> WNSRYSYNQLKNKDSLIMFLVEIFRSLFVSNCIDKNIDNVLLSIEEMFIDHYYNPQHSRLKYLIDDVGIFFTKLPITKAFHTYNKKYRITKRLYAPPTFNEVRHILNLAQILSLEEGLDLLTFDANETLYPDGHDFNDEVLASYISCLLKKMNIAIVTAASYNNDAEKYQKRLENLLKYFSKHNIKDGSYKNFYVMGGESNYLFKCNEEATL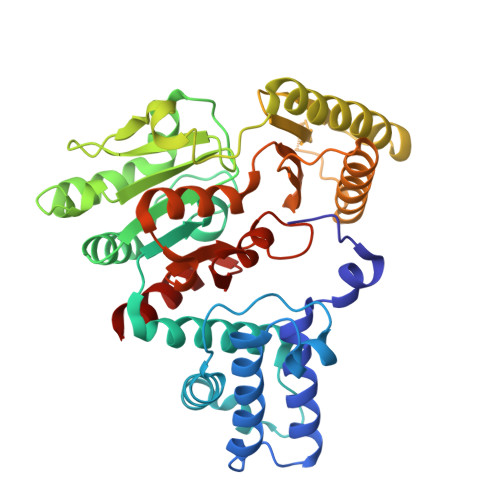YSVPENEWRHYKKFVDYDTVQEILNISEKCLEKVIKDFGLCAQIQRKEKSIGLVPNKIPSLNIKNEQKNYMIKYEVLEEAVIRIKKEIIKNKITAPYCAFNGGQDLWVDVGNKAEGLLILQKLLKIQKKKCCHIGDQFLHSGNDFPTRFCSLTLWVSNPQETKACLKSIMHL>[6x]MRGSHHHHHHGSMDKNIIIGAMTALITPFKNGKVDEQSYARLIKRQIENGIDAVVPVGTTGESATLTHEEHRTCIEIAVETCKGTKVKVLAGAGSAATHEAVGLAKFAKEHGADGILSV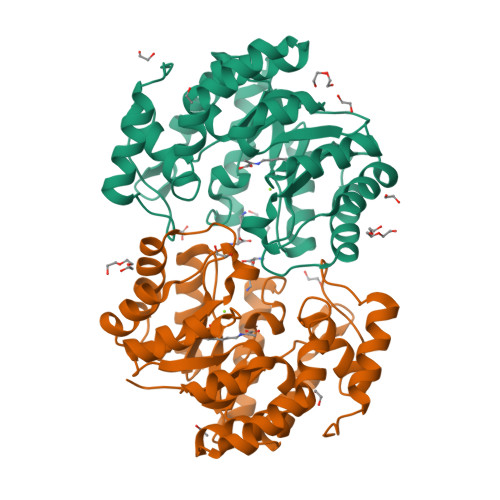APYYNKPTQQGLYEHYKAIAQSVDIPVLLYNVPGRTGCEISTDTIIKLFRDCENIYGVKEASGNIDKCVDLLAHEPRMMLISGEDAINYPILSNGGKGVISVTSNLLPDMISALTHFALDENYKEAKKINDELYNINKILFCESNPIPIKTAMYLAGLIESLEFRLPLCSPSKENFAKIEEVMKKYKIKGF> KPKLLNKFDKTIKAELDAAEKLRKRGKIEEAVNAFKELVRKYPQSPRARYGKAQCEDDLAEKRRSNEVLRGAIETYQEVASLPDVPADLLKLSLKRRSDRQQFLGHMRGSLLTLQRLVQLFPNDTSLKNDLGVGYLLIGDNDNAKKVYEEVLSVTPNDGFAKVHYGFILKAQNKIAESIPYL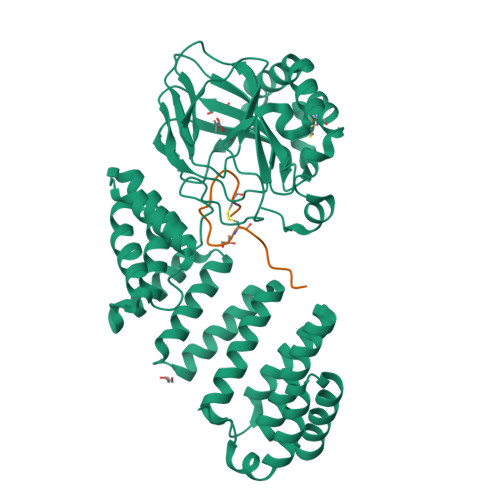KEGIESGDPGTDDGRFYFHLGDAMQRVGNKEAYKWYELGHKRGHFASVWQRSLYNVNGLKAQPWWTPKETGYTELVKSLERNWKLIRDEGLAVMDKAKGLFLPEDENLREKGDWSQFTLWQQGRRNENACKGAPKTCTLLEKFPETTGCRRGQIKYSIMHPGTHVWPHTGPTNCRLRMHLGLVIPKEGCKIRCANETKTWEEGKVLIFDDSFEAEVWQDASSFRLIFIVDVWHPELTPQQRRSLPAI;> DGDQSETSPSQNQGKCKDGLGEYTCTSLEGFEGKNSELF>MFEIKKICCIGAGYVGGPTCSVIAHMCPEIRVTVVDVNESRINAWNSPTLPIYEPGLKEVVESCRGKNLFFSTNIDDAIKEADLVFISVNTPTETYGMGKGRAADLKYIEACARRIVQNSNGYKIVTEKSTVPVRAAESIRRIFDANTKPNLNLQVLSNPEFLAEGTAIKDLKNPDRVLIGGDETPEGQRAVQALCAVYEHWVPREKILTTNTWSSELSKLAANAFLAQRISSINSISALCEATGADVEEVATAIGMDQRIGNKFLKASVGFGGSCFQKDVLNLVYLCEALNLPEVARYWQQVIDMNDYQRRRFASRIIDSLFNTVTDKKIAILGFAFKKDTGDTRESSSIYISKYLMDEGAHLHIYDPKVPREQIVVDLSHPGVSEDDQVSRLVTISKDPYEACDGAHAVVICTEWDMFKELDYERIHKKMLKPAFIFDGRRVLDGLHNELQTIGFQIETIGKKVSSKRIPYAPSGEIPKFSLQDPPNK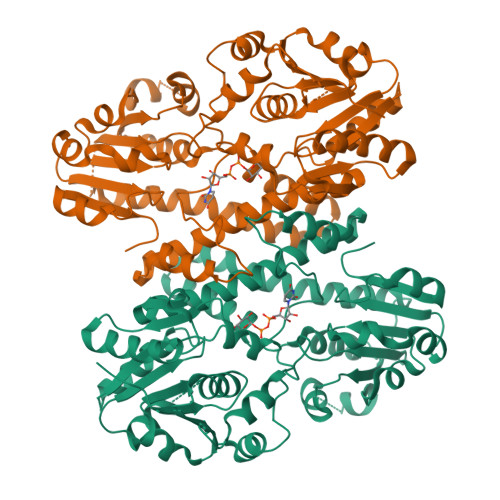KPKV[4x]> AGHHHHHHEETLLNTKLETADLKWVTFPQVDGQWEELSGLDEEQHSVRTYEVCDVQRAPGQAHWLRTGWVPRRGAVHVYATLRFTMLECLSLPRAGRSCKETFTVFYYESDADTATALTPAWMENPYIKVDTV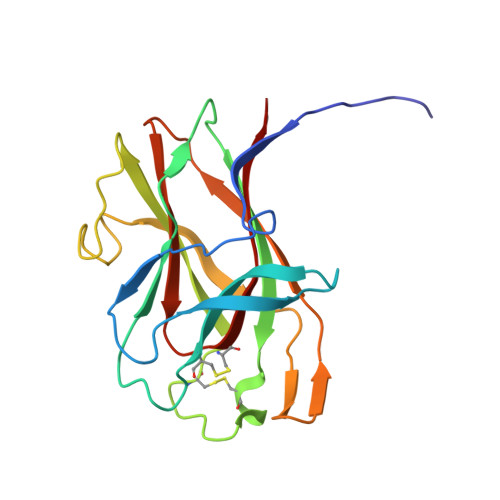AAEHLTRKRPGAEATGKVNVKTLRLGPLSKAGFYLAFQDQGACMALLSLHLFYKK>AMENKIEVNNKDEMNRWFEEFKKGNGLVDTFTNSYSFCESVPNLDRFVFQMASATDDAQKDSIYASALVEATKFCAPIYECAWVSSTGIVKKGLEWFEKNAGTIKSWDESYTELKVDVPKIEQLTGYQQAALKWRKDIGFRVNANTAALSNKVLAEYKVPGEIVMSVKEMLSDMIRRRNLILNRGGDENPRGPVSHEHVDWCREFVKGKYIMAFNPPWGDINKSGRSGIALVATGLAKLAETEGKGIFDEAKKTVEALNGYLDKHKDEVDRASADSMITNLLKHIAKAQELYKNSSALRAQSAQIDTAFSSYYWLYKAGVTPETFPTVSQFLFELGKQPRGTKKMKKALLSTPMKWGKKLYELFADDSFQQNRIYMHPAVLTAGRISEMGVCFGTIPVANPDDAAQGSGHTKSILNLRTNTETNNPCAKTIVKLFEVQKTGFNIQDMDIVASEHLLHQSLVGKQSPFQNAYNVKGNATSANII[2x];> AMENKIEVNNKDEMNRWFEEFKKGNGLVDTFTNSYSFCESIPNLDRFVFQMASATDDAQKDSIYASALVEATKFCAPIYECAWVSSTGIVKKGLEWFEKNAGTIKSWDESYTELKVDVPKIEQLTGYQQAALKWRKDIGFRVNANTAALSNKVLAEYKVPGEIVMSVKEMLSDMIRRRNLILNRGGDENPRGPVSHEHVDWCREFVKGKYIMAFNPPWGDINKSGRSGIALVATGLAKLAETEGKGIFDEAKKTVEALNGYLDKHKDEVDRASADSMITNLLKHIAKAQELYKNSSALRAQSAQIDTAFSSYYWLYKAGVTPETFPTVSQFLFELGKQPRGTKKMKKALLSTPMKWGK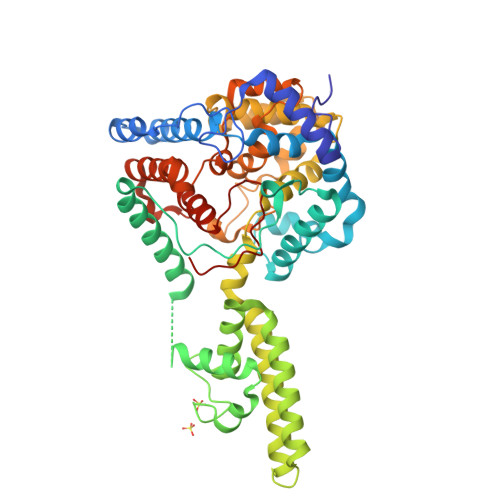KLYELFADDSFQQNRIYMHPAVLTAGRISEMGVCFGTIPVANPDDAAQGSGHTKSILNLRTNTETNNPCAKTIVKLFEVQKTGFNIQDMDIVASEHLLHQSLVGKQSPFQNAYNVKGNATSANII GERMACRENE A | C15 H24 | 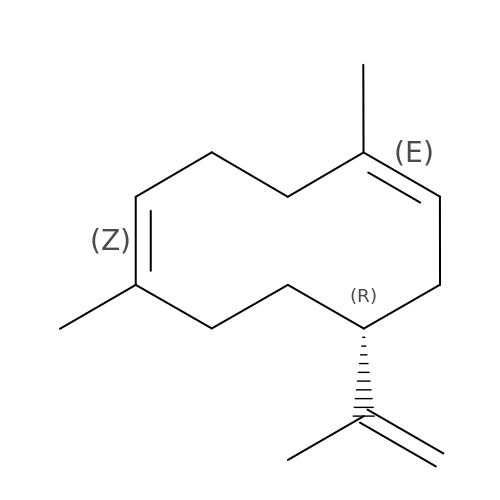XMRKUJJDDKYUHV-OAHLLOKOSA-N>MSLSKKTIYIAGLGLIGGSLALGIKRDHPDYEILGYNRSDYSRNIALERGIVDRATGDFKEFAPLADVIILAVPIKQTMAYLKELADLDLKDNVIITDAGSTKREIVEAAERY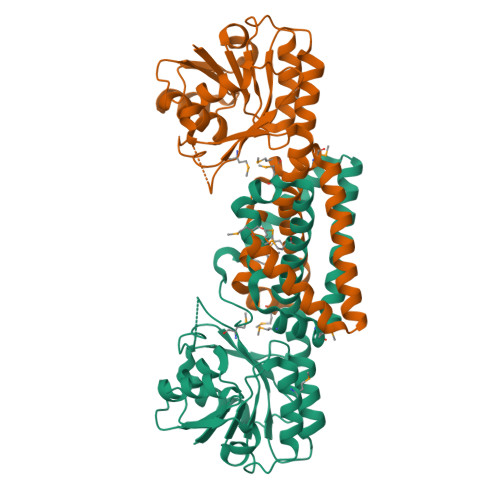LTGKNVQFVGSHPMAGSHKSGAIAADVTLFENAYYIFTPTSLTKETTIPELKDILSGLKSRYVEIDAAEHDRVTSQISHFPHLLASGLMEQAADYAQAHEMTNHFAAGGFRDMTRIAESEPGMWASILMTNGPAVLDRIEDFKKRLDHVADLIKAEDESAIWEFFDNGRKKRKEMEIHKKGGVESAFDIFVDVPDREGHHHHHH[2x]> MAQPFAWQVASLADRYEESFDIGAAVEPHQLNGRQGKVLKHHYNSIVAENAMKPISLQPEEGVFTWDGADAIVEFARKNNMNLRFHTLVWHNQVPDWFFLDEEGNPMVEETNEAKRQANKELLLERLETHIKTVVER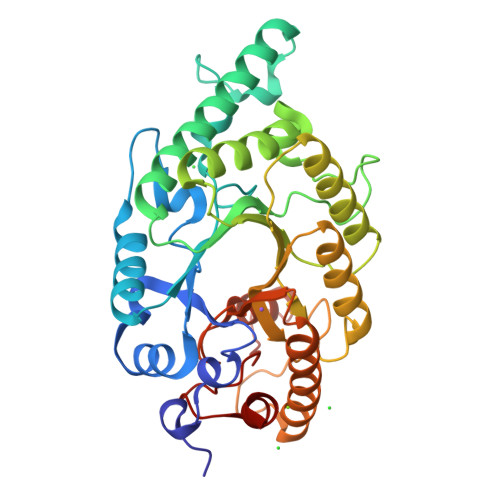YKDDVTAWDVVNEVVDDGTPNERGLRESVWYQITGDEYIRVAFETARKYAGEDAKLFINDYNTEVTPKRDHLYNLVQDLLADGVPIDGVGHQAHIQIDWPTIDEIRTSMEMFAGLGLDNQVTELDVSLYGWPPRPAFPTYDAIPQERFQAQADRYNQLFELYEELDADLSSVTFWGIADNHTWLDDRAREYNDGVGKDAPFVFDPNYRVKPAFWRIID(3AR,5R,6S,7R,7AR)-5-(HYDROXYMETHYL)-2-PROPYL-5,6,7,7A-TETRAHYDRO-3AH-PYRANO[3,2-D][1,3]THIAZOLE-6,7-DIOL 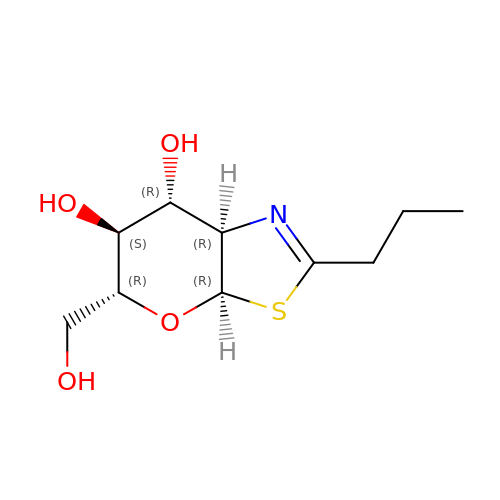| C10 H17 N O4 S | QWOPEBCGKASVQP-QXOHVQIXSA-N>QQSLAVKTFEDLFAELGDRARTRPADSTTVAALDGGVHALGKKLLEEAGEVWLAAEHESNDALAEEISQLLYWTQVLMISRGLSLDDVYR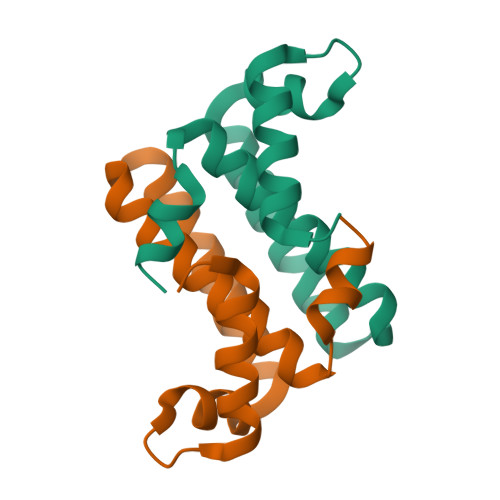KL[4x]However, because PPi is stable under normal conditions, inorganic pyrophosphatase (PPase) has evolved to specifically hydrolysis the molecule. Here, we solved four crystal structures of a family I type PPase from a strain of the pathogen Acinetobacter baumannii. The crystal structures of AbPPase showed that the enzyme has a typical Rossman fold domain that is highly conserved compared to other PPases. Family I PPases are hexamers formed by two stacks of trimers.

In Structure 1, we identified not only one Mg2+ (M1) bound to the catalytic center, but also a Na+ bound to a loop (residue 143–149) close to the catalytic center. The space group of Structure 1 is P6322, and there is only one AbPPase monomer in the asymmetric unit. This indicates that all monomeric AbPPases have the same structure. In AbPPase, β-ketone groups from two highly conserved residues, Lys143 and Lys149, coordinate with this Na+. Moreover, Pro147 forms the turn of that loop. Since this loop is close to the catalytic center, this Na+ might regulate hydrolysis activity by modifying the conformation of the loop. We found that the presence of Na+ could attenuate the hydrolytic activity of AbPPase. The elution profiles of AbPPase in these running buffers are the same, indicating that the inhibitory effects of Na+ occur via binding to the loop, rather than by altering the global structure of the enzyme. Structural and biochemical analysis of apo AbPPase shows that the binding of a Na+ ion to residues within a loop close to the catalytic center could inhibit the enzyme reaction.

> GSHMSYNNIPAGKDAPNDIYVIIEIPANAAPIKYEIDKDSDALFVDRFMGTAMFYPANYGYVPNTLSEDGDPLDVLVVTPYPVAAGSVIRCRPVGKLNMEDDGGIDAKLIAVPHEKLSPLYKDVKEYTDLPQLLINQVEHFFSHYKDLEPGKWVKISGWEGADVAKAEVIKAIEAAK>[2x]MSLKTTEYVAEILNELHNSAAYISNEEADQLADHILSSHQIFTAGAGRSGLMAKSFAMRLMHMGFNAHIVGEILT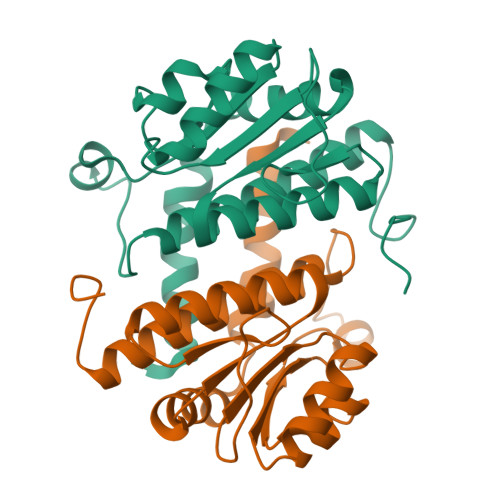PPLAEGDLVIIGSGSGETKSLIHTAAKAKSLHGIVAALTINPESSIGKQADLIIRMPGSPKDQSNGSYKTIQPMGSLFEQTLLLFYDAVILKLMEKKGLDSETMFTHHANLEEGGSHHHHHH N-{(1S)-5-{[2-(methylsulfanyl)benzene-1-carbonyl]amino}-1-[5-(naphthalen-2-yl)-1H-imidazol-2-yl]pentyl}-1,3-thiazole-5-carboxamide | C30 H29 N5 O2 S2 | 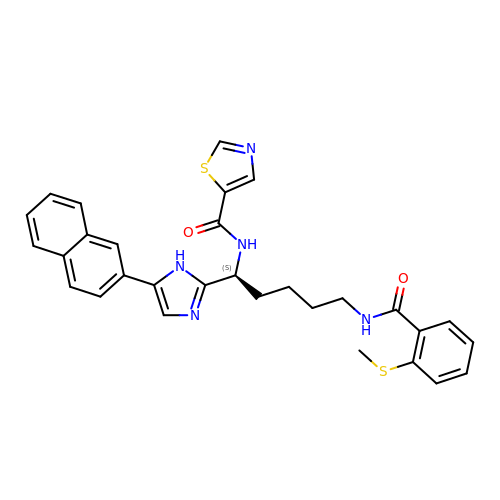IBVNIPPBTCWYJG-DEOSSOPVSA-N> TSF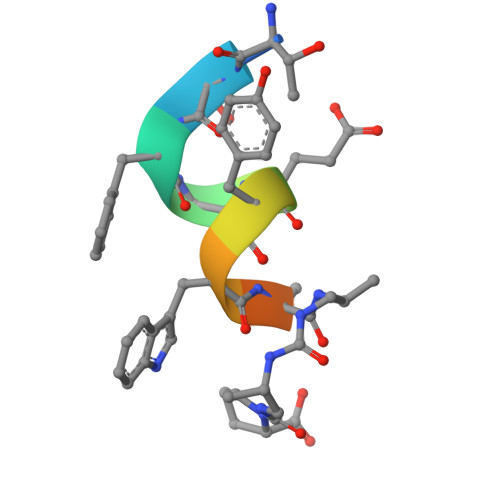AEYWAXXP>MTTATAGLAVELKQSTAQACEKAEHSTFMSDLLKGRLGVAEFTRLQEQAWLFYTALEQAVDAVRASGFAESLLDPALNRAEVLARDLDKLNGSSEWRSRITASPAVIDYVNRLEEIRDNVDGPALVAHHYVRYLGDLSGGQVIA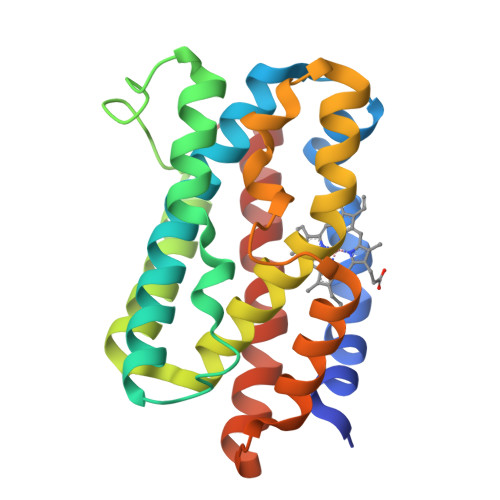RMMQRHYGVDPEALGFYHFEGIAKLKVYKDEYREKLNNLELSDEQREHLLKEATDAFVFNHQVFADLGKGL[2x]Here we report a detailed structure-function analysis of the kinase ThiM, which phosphorylates THZ in one of the first steps in vitamin B1 biosynthetic pathway. The quaternary structure of SaThiM is a triangular homo-trimer with dimensions of approximately 72 Å on a side and 47 Å thick with three independent active sites, each located within interface regions between two monomers. The following β-sheet strand 7 is antiparallel to strand 6 and following β-sheet strand 8, which is antiparallelly flanked by β-sheet strand 9. This fold of the phosphotransferase ThiM is homologous to that common to the group of ribokinase-like folded kinases. The three active sites, each located within the interface regions of two monomers respectively, are homologous to other known phosphoryl transfer ribokinase-like kinases.

In an attempt to achieve a maximum in accuracy and reliability of the structure, micro crystals grown under microgravity conditions onboard Chinese space mission Shenzhou-815 were used to prepare seed stock solutions to grow crystals suitable for X-ray diffraction. We observed an increase in crystal quality compared to native triclinic SaThiM crystals obtained in previous experiments. The structure of native SaThiM was solved and refined to 2.1 Å resolution with R and Rfree values of 20.34% and 23.04% respectively. The homologue structure of Bacillus subtilis ThiK (PDB code: 1C3Q19), sharing 38% sequence identity, was used as a search model for molecular replacement phasing. The core of each monomer contains nine β-sheets that are flanked by five α-helices and six α-helices. For all six molecules in the asymmetric unit no electron density was observed for the last two residues of the C-terminus and for the loop region between residues 126 and 140. Therefore these residues were not modeled. Analysing the interface regions of protomers A, B and C revealed that 10 intermolecular H-bonds support the complex formation. No Mg2+ ion was found in the native structure.

>MNYLNNIRIENPLTICYTNDVVKNFTANGLLSIGASPAMSEAPEEAEEFYKVAQALLINIGTLTAQNEQDIIAIAQTANEAGLPIVFDPVAVGASTYRKQFCKLLLKSAKVSVIKGNASEILALIDDTATMKGTDSDANLDAVTIAKKAYAIYKTAIVITGKEDVIVQGDKAIVLANGSPLLARVTGAGCLLGGIIAGFLFRETEPDIEALIEAVSVFNIAAEVAAENENCGGPGTFSPLLLDTLYHLNETTYQQRIRIQEVEENLYFQSGHHHHHH[6x]> MFLKRLDVIGFKSFAERISVDFVKGVTAVVGPNGSGKSNITDAIRWVLGEQSARSLRGGKMEDIIFAGSDSRKRLNLAEVTLTLDNDDHFLPIDFHEVSVTRRVYRSGESEFLINNQPCRLKDIIDLFMDS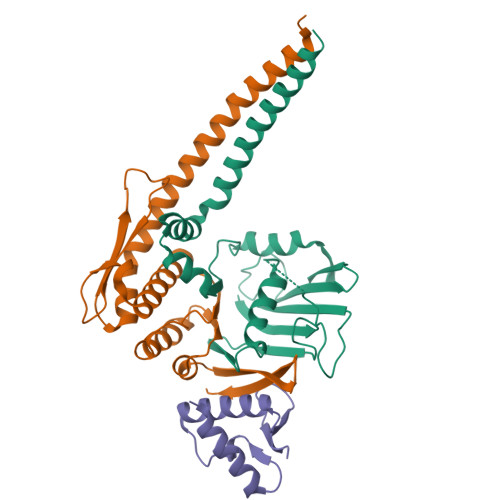GLGKEAFSIISQGKVEEILSSKAEDRRSIFEEAAGVLKYKTRKKKAENKLFETQDNLNRVEDILHELE;> MRYKFLSEQKEDLTEAKNTLFQVIEEMDEEMTKRFNDTFVQIRSHFDQVFRSLFGGGRAELRLTDPNDLLHSGVEIIAQPPGKKLQNLNLLSGGERALTAIALLFSILKVRPVPFCVLDQVEAALDEANVFRFAQYLKKYSSDTQFIVITHRKGTMEEADVLYGVTMQESGVSKVISVKLEETKEFVQ;> GPHMRQDIPIEARMNEIVHSLKSRGTRINFMDLFPYEQKEHLVVTFLAVLELMKNQLVLIEQEHNFSDIYITGSESIHGA>[3x]GSHMTKITLSDLPLREELRGEHAYGAPQLNVDIRLNTNENPYPPSEALVADLVATVDKIATELNRYPERDAVELRDELAAYITKQTGVAVTRDNLWAANGSNEILQQLLQAFGGPGRTALGFQPSYSMHPILAKGTHTEFIAVSRGADFRIDMDVALEEIRAKQPDIVFVTTPN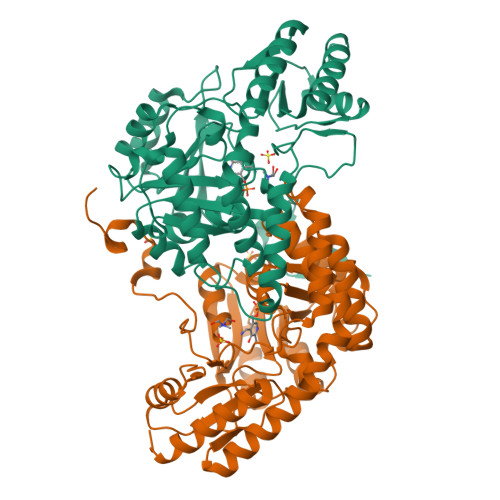NPTGDVTSLDDVERIINVAPGIVIVDEAYAEFSPSPSATTLLEKYPTKLVVSRTMSKAFDFAGGRLGYFVANPAFIDAVMLVRLPYHLSALSQAAAIVALRHSADTLGTVEKLSVERVRVAARLEELGYAVVPSESNFVFFGDFSDQHAAWQAFLDRGVLIRDVGIAGHLRTTIGVPEENDAFLDAAAEIIKLNL>[2x]KTPDMGSFHADMGSCQSCHAKPIKVTDSETHENAQCKSCHGEYAELANDKLQFDPHNSHLGDINCTSCHKGHEEPKFYCNECHSFDIKPMPFSDAKKKKSWDDGWDQDKIQKAIAAGPSETTQVLVVGAGSAGFNASLAAKKAGANVILVDKAPFSGGNSMISAGGMNAVGTKQQTAHGVEDKVEWFIEDAMKGGRQQNDIKLVTILAEQSADGVQWLESLGANLDDLKRSGGARVDRTHRPHGGKSSGPEIIDTLRKAAKEQGIDTRLNSRVVKLVVNDDHSVVGAVVHGKHTGYYMIGAKSVVLATGGYGMNKEMIAYYRPTMKDMTSSNNITATGDGVLMAKEIGAS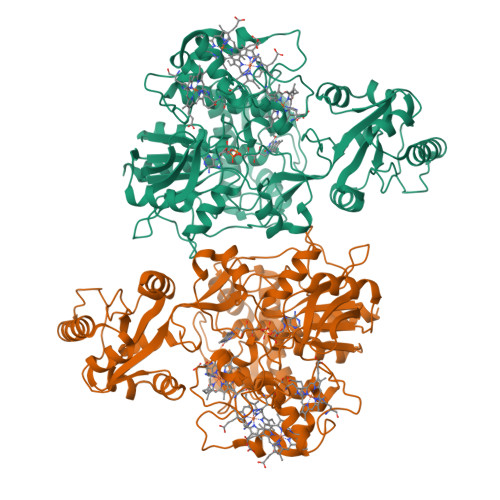MTDIDWVQAHPTVGKDSRILISETVRGVGAVMVNKDGNRFISELTTRDKASDAILKQPGQFAWIIFDNQLYKKAKMVRGYDHLEMLYKGDTVEQLAKSTGMKVADLAKTVSDYNGYVASGKDTAFGRADMPLNMTQSPYYAVKVAPGIHHTMGGVAINTTASVLDLQSKPIDGLFAAGEVTGGVHGYNRLGGNAIADTVVFGRIAGDNAAKHALDK> QHRSRSESSIESFFARGACVTIMTVDNPASTTNKDKLFAVWKITYKDTVQLRRKLEFFTYSRFDMELTFVVTANFTETNNGHALNQVYQIMYVPPGAPVPEKWDDYTWQTSSNPSIFYTYGTAPARISVPYVGISNAYSHFYDGFSKVPLKDQSAALGDSLYGAASLNDFGILAVRVVNDHNPTKVTSKIRVYLKPKHIRVWCPRPPRAVAYYGPGVDYKDGTLTPLSTKDLTTY;> LQLTLGNSTITTQE;> GLPVMNTPGSNQYLTADNFQSPCALPEFDVTPPIDIPGEVKNMMELAEIDTMIPFDLSATKKNTMEMYRVRLSDKPHTDDPILCLSLSPASDPRLSHTMLGEILNYYTHWAGSLKFTFLFCGSMMATGKLLVSYAPPGADPPKKRKEAMLGTHVIWDIGLQSSCTMVVPWISNTTYRQTIDDSFTEGGYISVFYQTRIVVPLSTPREMDILGFVSACNDFSVRLLRDTTHI;> AANSVVAYGRWPEYLRDSEANPVDQPTEPDVAACRFYTLDTVSWTKESRGWWWKLPDALRDMGLFGQNMYYHYLGRSG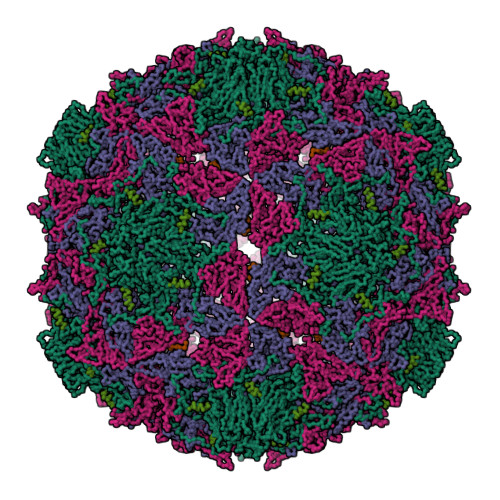YTVHVQCNASKFHQGALGVFAVPEMCLAGDSNTTTMHTSYQNANPGEKGGTFTGTFTPDNNQTSPARRFCPVDYLLGNGTLLGNAFVFPHQIINLRTNNCATLVLPYVNSLSIDSMVKHNNWGIAILPLAPLNFASESSPEIPITLTIAPMCCEFNGLRNITLPRLQ>[4x]SNASAAEAPLPQLRAYTVDASWLQPMAPLQVADHTWQIGTEDLTALLVQTAEGAVLLDGGMPQMAGHLLDNMKLRGVAPQDLRLILLSHAHADHAGPVAELKRRTGAHVAANAETAVLLARGGSNDLHFGDGITYPPASADRIIMDGEVVTVGGIAFTAHFMPGHTPGST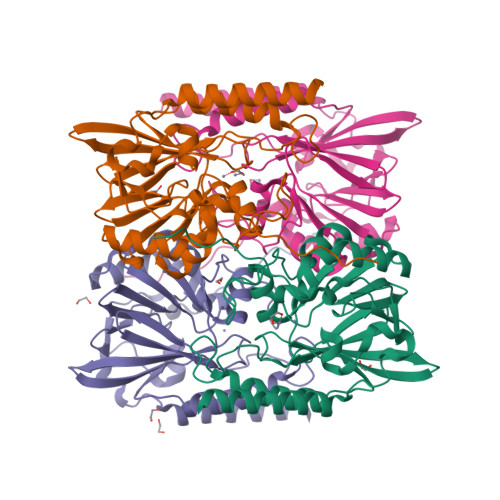AWTWTDTRDGKPVRIAYADSLSAPGYQLKGNPRYPRLIEDYKRSFATVRALPCDLLLTPHPGASNWNYAVGSKASAEALTCNAYADAAEKKFDAQLARETAGTR> MSAEAADREAATSSRPCTPPQTCWFEFLLEESLLEKHLRKPCPDPAPVQLIVQFLEQASKPSVNEQNQVQPPPDNKRNRILKLLALKVAAHLKWDLDILEKSLSVPVLNMLLNELLCISKVPPGTKHVDMDLATLPPTTAMAVLLYNRWAIRTIVQSSFPVKQAKPGPPQLSVMNQMQQEKELTENILKVLKEQAADSILVLEAALKLN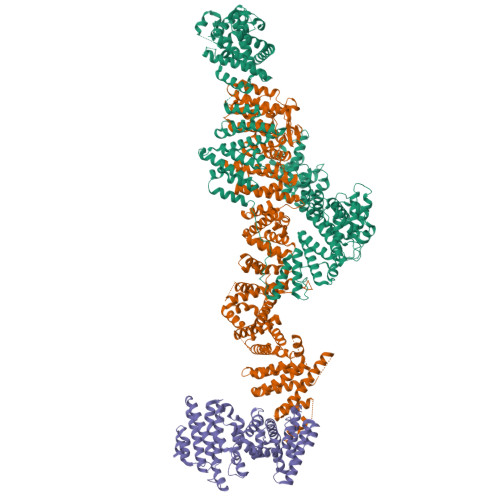KDLYVHTMRTLDLLAMEPGMVNGETESSTAGLKVKTEEMQCQVCYDLGAAYFQQGSTNSAVYENAREKFFRTKELIAEIGSLSLHCTIDEKRLAGYCQACDVLVPSSDSTSQQLTPYSQVHICLRSGNYQEVIQIFIEDNLTLSLPVQFRQSVLRELFKKAQQGNEALDEICFKVCACNTVRDILEGRTISVQFNQLFLRPNKEKIDFLLEVCSRSVNLEKASESLKGNMAAFLKNVCLGLEDLQYVFMISSHELFITLLKDEERKLLVDQMRKRSPRVNLCIKPVTSFYDIPASASVNIGQLEHQLILSVDPWRIRQILIELHGMTSERQFWTVSNKWEVPSVYSGVILGIKDNLTRDLVYILMAKGLHCSTVKDFSHAKQLFAACLELVTEFSPKLRQVMLNEMLLLDIHTHEAGTGQAGERPPSDLISRVRGYLEMRLPDIPLRQVIAEECVAFMLNWRENEYLTLQVPAFLLQSNPYVKLGQLLAATCKELPGPKESRRTAKDLWEVVVQICSVSSQHKRGNDGRVSLIKQRESTLGIMYRSELLSFIKKLREPLVLTIILSLFVKLHNVREDIVNDITAEHISIWPSSIPNLQSVDFEAVAITVKELVRYTLSINPNNHSWLIIQADIYFATNQYSAALHYYLQAGAVCSDFFNKAVPPDVYTDQVIKRMIKCCSLLNCHTQVAILCQFLREIDYKTAFKSLQEQNSHDAMDSYYDYIWDVTILEYLTYLHHKRGETDKRQIAIKAIGQTELNASNPEEVLQLAAQRRKKKFLQAMAKLYF;> MSALCDPPGAPGPPGPAPATHGPAPLSAQELSQEIKAFLTGVDPILGHQLSAREHARCGLLLLRSLPPARAAVLDHLRGVFDESVRAHLAALDETPVAGPPHLRPPPPSHVPAGGPGLEDVVQEVQQVLSEFIRANPKAWAPVISAWSIDLMGQLSSTYSGQHQRVPHATGALNELLQLWMGCRATRTLMDIYVQCLSALIGSCPDACVDALLDTSVQHSPHFDWVVAHIGSSFPGTIISRVLSCGLKDFCVHGGAGGGAGSSGGSSSQTPSTDPFPGSPAIPAEKRVPKIASVVGILGHLASRHGDSIRRELLRMFHDSLAGGSGGRSGDPSLQATVPFLLQLAVMSPALLGTVSGELVDCLKPPAVLSQLQQHLQGFPREELDNMLNLAVHLVSQASGAGAYRLLQFLVDTAMPASVITTQGLAVPDTVREACDRLIQLLLLHLQKLVHHRGGSPGEGVLGPPPPPRLVPFLDALKNHVGELCGETLRLERKRFLWQHQLLGLLSVYTRPSCGPEALGHLLSRARSPEELSLATQLYAGLVVSLSGLLPLAFRSCLARVHAGTLQPPFTARFLRNLALLVGWEQQGGEGPAALGAHFGESASAHLSDLAPLLLHPEEEVAEAAASLLAICPFPSEALSPSQLLGLVRAGVHRFFASLRLHGPPGVASACQLLTRLSQTSPAGLKAVLQLLVEGALHRGNTELFGGQVDGDNETLSVVSASLASASLLDTNRRHTAAVPGPGGIWSVFHAGVIGRGLKPPKFVQSRNQQEVIYNTQSLLSLLVHCCSAPGGTECGECWGAPILSPEAAKAVAVTLVESVCPDAAGAELAWPPEEHARATVERDLRIGRRFREQPLLFELLKLVAAAPPALCYCSVLLRGLLAALLGHWEASRHPDTTHSPWHLEASCTLVAVMAEGSLLPPALGNMHEVFSQLAPFEVRLLLLSVWGFLREHGPLPQKFIFQSERGRFIRDFSREGGGEGGPHLAVLHSVLHRNIDRLGLFSGRFQAPSPSTLLRQGT;> MSDIRHSLLRRDALSAAKEVLYHLDIYFSSQLQSAPLPIVDKGPVELLEEFVFQVPKERSAQPKRLNSLQELQLLEIMCNYFQEQTKDSVRQIIFSSLFSPQGNKADDSRMSLLGKLVSMAVAVCRIPVLECAASWLQRTPVVYCVRLAKALVDDYCCLVPGSIQTLKQIFSASPRFCCQFITSVTALYDLSSDDLIPPMDLLEMIVTWIFEDPRLILITFLNTPIAANLPIGFLELTPLVGLIRWCVKAPLAYKRKKKPPLSNGHVSNKVTKDPGVGMDRDSHLLYSKLHLSVLQVLMTLQLHLTEKNLYGRLGLILFDHMVPLVEEINRLADELNPLNASQEIELSLDRLAQALQVAMASGALLCTRDDLRTLCSRLPHNNLLQLVISGPVQQSPHAALPPGFYPHIHTPPLGYGAVPAHPAAHPALPTHPGHTFISGVTFPFRPIR Nalpha-[(3-tert-butyl-1-methyl-1H-pyrazol-5-yl)carbonyl]-N-[(2E)-2-iminoethyl]-3-{5-[(Z)-iminomethyl]-1,3,4-oxadiazol-2-yl}-L-phenylalaninamide 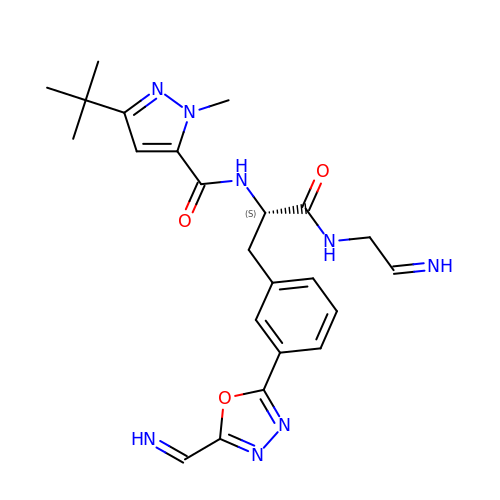| C23 H28 N8 O3 | TVWDSIGUOHNHHP-TTWIPJPDSA-N> MRKLYLFLFLTLISPISISIFHAQCTGATVESLTNPGPYTVATLSEADGVRNGPKYAGSTIYYPTNATPPYASIAIVPGFTAAPSSVQEWGPFYASHGIVAIIIGTNSLYDQPEARALALLDALETIKQENGRATSPLIGKLDVTKLAVSGWSMGGGGAQRAAVLDNTISAVVALCPYLTSPQLNHTVPVLIFSGQSDPTAPPSQHANVHYNTTPGTTNKLLFEVKNGNHSVANSPTGGGGAVGKLALSWLKIYLEKNDCYCSVLATAIVNSTTVSSKISQSYQCNNALGVVDSKTRFNLYPNPTKDFVQVNVREMASYQLSSSTGQIVLKGIVTSSKNQIDLSKLPAGVYYLQINGETIKVIKKQ

Here, we describe the first functional PET-active enzymes from the Bacteroidetes phylum. Among them, two promiscuous and cold-active esterases derived from Aequorivita sp. (PET27) and Kaistella jeonii (PET30) showed depolymerizing activity on polycaprolactone (PCL), amorphous PET foil and on the polyester polyurethane Impranil® DLN. PET30, annotated as a potential lipase, was derived from the published genome sequence of Kaistella jeonii NCTC 13459. The enzymes PET27 and PET30 characterized here are both typical esterases (i.e., serine hydrolases) belonging to the EC 3.1.

To ensure that this C-terminus does not affect catalytic activity, a deletion mutant designated PET30ΔPorC was created that lacked the sorting sequence between the amino acids 300–366. Activity tests confirmed that it was not affected in its activities using pNP-C6 or PET foil. The crystal structure of PET30 without its C-terminal Por-domain (PET30ΔPorC) was solved at 2.1 Å and displays high structural similarity to the IsPETase. The structure was solved at 2.1 Å resolution, containing one monomer in the asymmetric unit, with 16.2% for Rwork and 21.9% for Rfree. The PET30ΔPorC protein shows a canonical α/β-fold consisting of a central twisted β-sheet composed of 9 β-strands flanked by 7 α-helices on both sides, as already reported for homologous structures, i.e., PETases and cutinases. The structure of PET30ΔPorC revealed an extra β-sheet (β10) which is located at the C-terminus and connects the PorC domain which has been deleted in this construct. PET30ΔPorC represents the overall fold of several PETases as revealed by a similarity search performed by PDBeFold. One disulfide bond is present in PET30ΔPorC (C262-C285), a common feature for Type II PET-degrading enzymes. Here similar interactions of the HEMT molecule by the PET30ΔPorC protein can be deduced mediated by Y178, T200, H230, W152, F80, and M154. PET30 shows a less hydrophobic surrounding of the catalytic pocket when compared to the structures of Type I and Type II PET-degrading enzymes.>[2x]MSMIKSYAAKEAGGELEVYEYDPGELRPQDVEVQVDYCGICHSDLSMIDNEWGFSQYPLVAGHEVIGRVVALGSAAQDKGLQVGQRVGIGWTARSCGHCDACISGNQINCEQGAVPTIMNRGGFAEKLRADWQWVIPLPENIDIESAGPLLCGGITVFKPLLMHHITATSRVGVIGIGGLGHIAIKLLHAMGCEVTAFSSNPAKEQEVLAMGADKVVNSRDPQALKALAGQFDLIINTV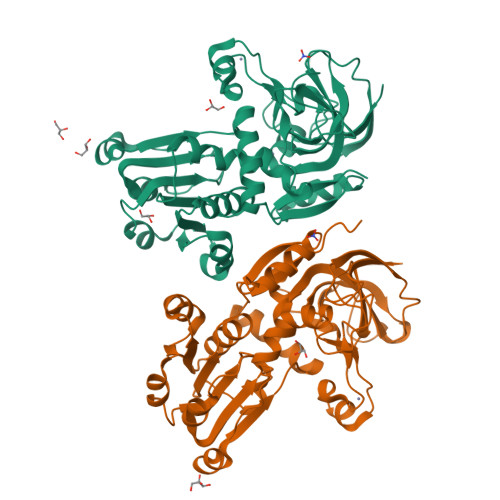NVSLDWQPYFEALTYGGNFHTVGAVLTPLSVPAFTLIAGDRSVSGSATGTPYELRKLMRFAARSKVAPTTELFPMSKINDAIQHVRDGKARYRVVLKADYLAHHHHHH>[2x]GSNAGGSSPITGLVYDQRMMLHHNMWDSHHPELPQRISRIFSRHEELRLLSRCHRIPARLATEEELALCHSSKHISIIKSSEHMKPRDLNRLGDEYNSIFISNESYTCALLAAGSCFNSAQAILTGQVRNAVAIVRPPGHHAEKDTACGFCFFNTAALTARYAQSITRE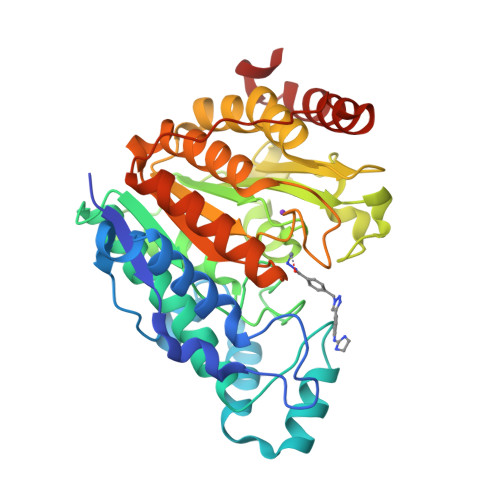SLRVLIVDWDVHHGNGTQHIFEEDDSVLYISLHRYEDGAFFPNSEDANYDKVGLGKGRGYNVNIPWNGGKMGDPEYMAAFHHLVMPIAREFAPELVLVSAGFDAARGDPLGGFQVTPEGYAHLTHQLMSLAAGRVLIILEGGYNLTSISESMSMCTSMLLGDSPPSLDHLTPLKTSATVSINNVLRAHAPFWSSLR>DSLKWIVFLQFLIVLLLLAIVFLLR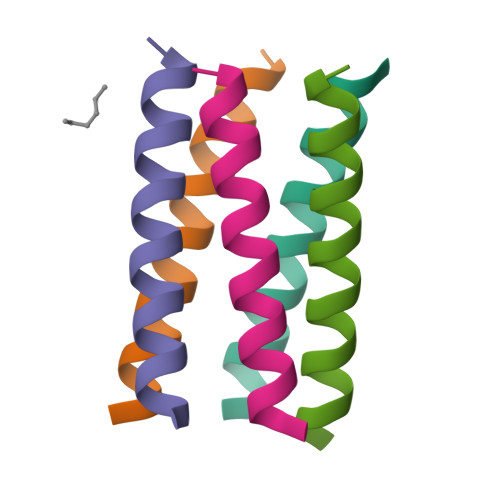G[10x]CI2 is a small single domain protein of 64 residues, which has been extensively used as a model to understand key concepts of protein folding and stability. L49 and I57 are both part of the folding nucleus in CI2 and very important for the stability of the folded state of CI232. Here, we have applied an efficient in-cell assay in E. coli to select variants of the barley chymotrypsin inhibitor 2 with increased stability. We, therefore, determined the crystal structures of all four CI2 variants in the wild-type to L49I/I57V double mutant cycle.

When wild-type CI2 is expressed in the bacterial sensor system only little GFP is produced. Analysis of the pairwise interaction energies at the residue level suggests that much of the stabilizing effect of the I57V mutation originates from an unfavourable interaction between I57 and Q59 that is observed in structures of both the wild-type and L49I. Previous stability studies of Ala mutants showed that there is strain in the native CI2 structure between I57 and A16 but not between L49 and A1640.

> MKTEWPELVGKSVEEAKKVILQDKPEAQIIVLPVGTIVTMEYRIDRVRLFVDKLDNIAQVPRVG> GAMDISQLFHDEVPLFDNSITSKDKEVIETLSEIYSIVITLDHVEKAYLKDSIDDTQYTNTVDKLLKQFKVYLNSQNKEEINKHFQSIEAFA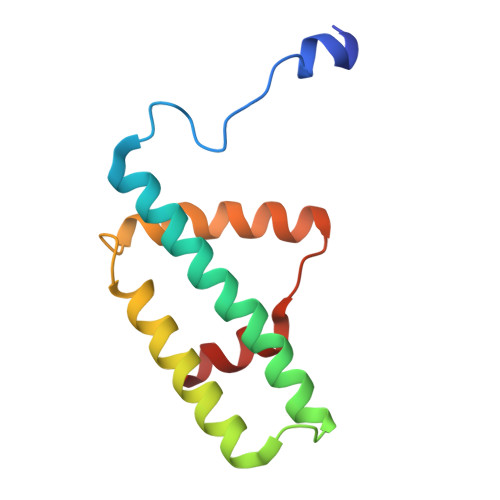DTYNITASNAITRLERG> MKSSHHHHHHENLYFQSNAEESAQQRSERYVSARSQHPAWLLLASRRAPLVLGCLRTLFERAHDGIPMEDALQALSEMLAAYASQELYEIDPDATHLQAGRELREWIKRRLVVEREGRIYATDALESAIQFVDSLDSRIMTSTASRLSVVQREIENLETGLNPSPTGRIASLRRRIQDLEHELARVEAGHVDVLDEAQAIEGMREVYNLATSLRADFRRVEDSWREADRALRHSIISEQSHRGEIVDRLLDGQDALLNTPEGRVFESFQQQLRQSAELEVMRERLRTILRHPAVPKALNRPQQRELRWLALRLVRESQAVLQARARSERDVRGFMKTGLAAEHHRVGQLLNDFFNLALSVDWQRQSERRKPACLPPVGVAITGVPAIERLRFKTLDDDDAGELDLSLKPAGLEQIDDDFWDAFDGLDREALIHDTLAVLVEQGRPVSLGELASLLPPAHDLETFALWLAMAREAG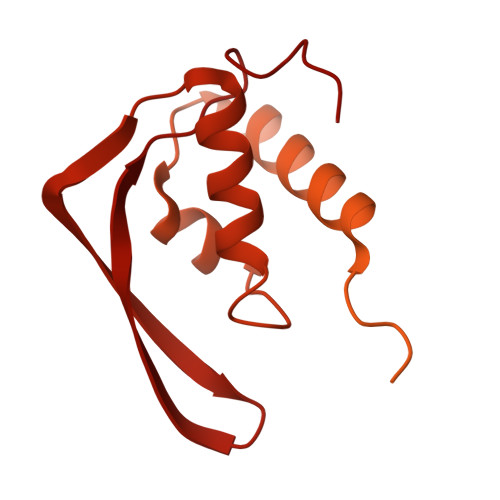IEVLTEERQFVELVDEDEQRWGFNLPYVGLDHEALKDIDWEL>[4x]MVDYSDCFEGISGGAIFYNTKNKEYNIYNKELIETRRSPCSTFKIVSTLIGLEKGVINSKESVMGYDGTEYPNKNWNKNLSLEEAFKESCVWYYKKLIDKVDAKSVQNILDD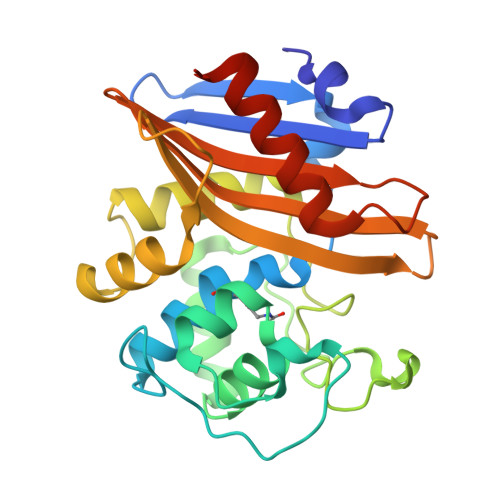LKYGNCDISEWEGDLKNGKGHLNGFWLESSLQISPKEQVQTMAKIFEGDTNFKKEHINILRDIMKIDVNDKNINVYGKTGTGFDEKNKRVDAWFVGMLEREGDTYYFAIKSDDSNKEITGPKVKEIAINIIKKYYSVREGAAL(3R,4S)-N-[2-chloro-5-(3-methoxypropyl)benzyl]-N-cyclopropyl-4-{4-[2-(2,6-dichloro-4-methylphenoxy)ethoxy]phenyl}piperidine-3-carboxamide | C35 H41 Cl3 N2 O4 | 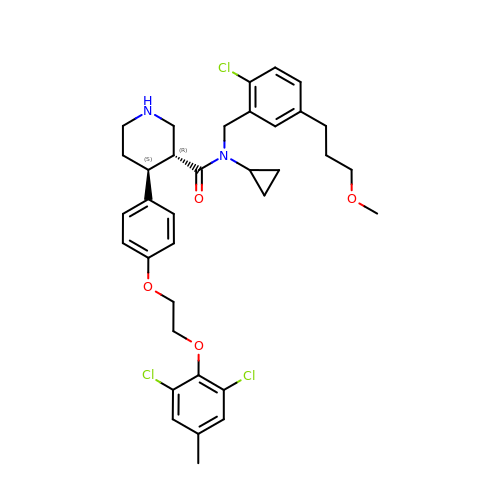RDCUZWVELSAOBC-IHLOFXLRSA-N2-O-{3-[AMINO(IMINO)METHYL]PHENYL}-5-O-{4-[AMINO(IMINO)METHYL]PHENYL}-1,4:3,6-DIANHYDRO-D-GLUCITOL 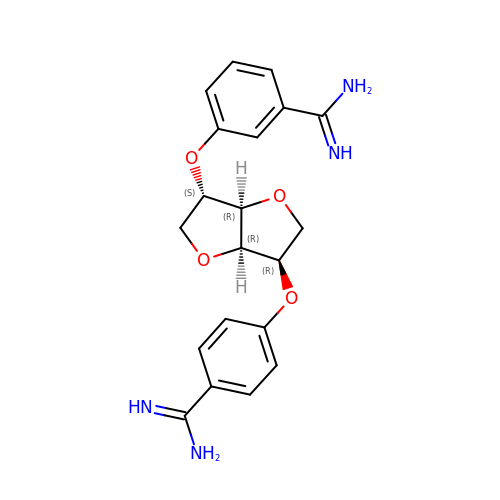| C20 H22 N4 O4 | DKBAWRNTUZFJKV-XMTFNYHQSA-N>TLIELMIVVAIIGILAAIAIPQYQNYIAKSQVSRVMSETGSLKTVIETCILDGKTAANCELGWTNSNLLG[22x];>STAAVTGQTGLTITYPASATESAAIQGTFGNSAAIKIKNQTLTWTRTPEGAWSCATTVEAKFKPAGCAS[22x]

Single-stranded RNA bacteriophages (ssRNA phages) are positive-sense RNA viruses that have shown specificity for gram-negative bacteria by exploiting host retractile pili, including T4P6. Acinetobacters have type IV pili (T4P), which are involved in twitching motility, surface adhesion, biofilm formation, and natural transformation in gram-negative bacteria. Our study delves into the interaction between Acinetobacter phage AP205 and type IV pili. Using cryo-electron microscopy, we solve structures of the AP205 virion with an asymmetric dimer of maturation proteins, the native Acinetobacter type IV pili bearing a distinct post-translational pilin cleavage, and the pili-bound AP205 showing its maturation proteins adapted to pilin modifications, allowing each phage to bind to one or two pili.

Using single-particle cryo-EM and helical reconstruction, we obtain a high-resolution structure of the purified straight T4P at 2.5 Å resolution and model the mature pilin into the cryo-EM density. The mature T4P pilin subunits have a distinct “lollipop” shape, presenting a globular C-terminal β-sheet domain and two N-terminal α-helices. They assemble into a 60Å-wide filament, with a helical rise of 10.0 Å and a twist angle of 91.9°. The β-sheet domain is exposed on the outside, while the α-helices are buried within the center of the filament. Within our helical reconstruction of A. gp16 T4P, additional density corresponding to potential glycans was observed. These glycans are added post-translationally to the last amino acid Ser147 of the mature pilin. Surprisingly, a 13-Å gap in the density of the polypeptide chain is observed between Gly78 and Ser79. This indicates that, in addition to the post-translational cleavage at the N-terminus to remove the signal peptide involving the first seven amino acids in the prepilin, there is another cleavage in the middle of the peptide chain, a phenomenon not reported for other pilins. While the precise mechanism behind such pilin cleavage remains undiscovered, the fact that it takes place on the external surface of T4P suggests a direct influence on its interactions with the environment, such as its engagements with the immune system or phages.Based on the structure-function knowledge of the RNase A superfamily we have engineered a chimera that combines RNase 1 highest catalytic activity with RNase 3 unique antipathogen properties. Based on the RNase 1 scaffold we incorporated specific regions essential for RNase 3 unique anti-pathogen activities within the RNase A superfamily. The solved crystal structures confirmed that all the chimera proteins reproduce the kidney-shaped folding typical of the RNase A superfamily and thus keep the fold of the templates used in their design, as suggested by circular dichroism and molecular dynamics analysis. Nonetheless, the structures that incorporated the key features related to RNase 3 antimicrobial activity retained the overall RNase 1 active site conformation together with the essential structural elements for binding to the human ribonuclease inhibitor (RNHI), ensuring non-cytotoxicity.

Last, a third version was designed, where the flexible loop L1 of RNase 1 was removed. Last, removal of an RNase 1 flexible loop (L1) in the third version enhanced its antimicrobial properties and catalytic efficiency. Finally, RNase 3/1-v3 was crystallized in the presence of phosphate anions. The structure has two molecules in the asymmetric unit with an RMSD between backbone chains of 0.27 Å. The C terminal β-strand is conserved in this version, keeping the geometry of the B1 pocket. While in RNase 3/1-v3 there is an extended β-strand, in the first two chimeras the C-terminus end is disordered, determining significant changes at the B1 pocket. Interestingly, an equivalent distribution of PO4 anions is obtained in RNase 3/1-v3, where phosphate n° 3 is located at the active site. In the case of RNase 3/1-v3, the replacement of the flexible loop of RNase 1 by the shorter and more rigid loop of RNase 3 reduces the capacity of the first two helixes to readapt the active site configuration, provoking a major displacement of both helixes and forming a hydrophobic core similar to RNase 3 one. In contrast, RNase 3/1-v3, thanks to the absence of the extended and more flexible L1 loop of RNase 1, might have a reduced protein motion and hence a reduced catalytic efficiency. Although the hinge residue His48 identified in the RNase A scaffold to mediate the protein motion is present in the three variants, this residue in the latest variant cannot perform equivalent interactions due to the absence of R1-L1. Two additional variants were later designed, where variant 3 combined the best of both parental proteins, achieving similar antimicrobial properties to RNase 3.

>[2x]MRPPQFTRAQWFAIQHISLNPPRCTIAMRAINNYRWRCKPVNTFVHEPLVDVQNVCFQEKVTCKNGQGNCYRSRFRMHITDCRLTNGSRYPNCRYRTRPGRRHIIVACENRDPRDSPRYPYVPVHFDASV> MPHTYEDPNQAVHEFAKEIE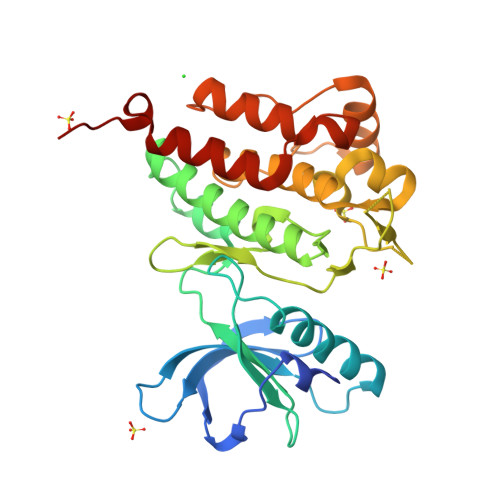ASCITIERVIGAGEFGEVCSGRLKLPGKRELPVAIKTLKVGYTEKQRRDFLGEASIMGQFDHPNIIHLEGVVTKSKPVMIVTEYMENGSLDTFLKKNDGQFTVIQLVGMLRGISAGMKYLSDMGYVHRDLAARNILINSNLVCKVSDFGLSRVLEDDPEAAYTTRGGKIPIRWTAPEAIAFRKFTSASDVWSYGIVMWEVVSYGERPYWEMTNQDVIKAVEEGYRLPSPMDCPAALYQLMLDCWQKERNSRPKFDEIVNMLDKLIRNPAHHHHHH>[2x]MGADDVVDSSKSFVMENFSSYHGTKPGYVDSIQKGIQKPKSGTQGNYDDDWEGFYSTDNKYDAAGYSVDNENPLSGKAGGVVKVTYPGLTKVLALKVDNAETIKKELGLSLTEPLMEQVGTEEFIKRFGDGASRVVLSLPFAEGSSSVKYINNWEQAKALSVELEINFETRGKRGQDAMYEYMAQACAGNRVRRSVGSSLSCINLDWDVIRDKTKTKIESLKEHGPIKNKMSESPNKTVSEEKAKQYLEEFHQTALEHPELSELKTVTGTNPVFAGANYAAWAVNVAQVIDSETADNLEKTTAALSILPGIGS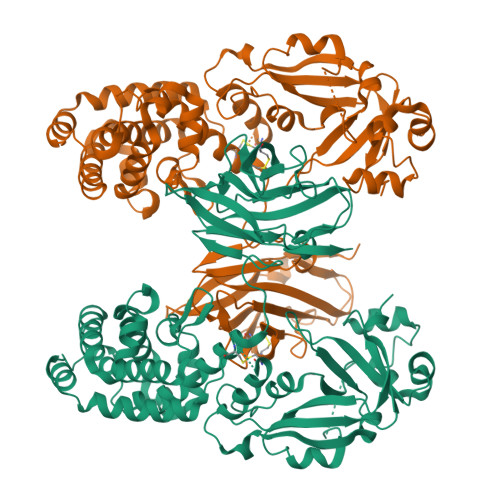VMGIADGAVHHNTEEIVAQSIALSSLMVAQAIPLVGELVDIGFAAYNFVESIINLFQVVHNSYNRPAYSPGHKTQPFLHDGYAVSWNTVEDSIIRTGFQGESGHDIKITAENTPLPIAGVLLPTIPGKLDVNKSKTHISVNGRKIRMRCRAIDGDVTFCRPKSPVYVGNGVHANLHVAFHRSSSEKIHSNEISSDSIGVLGYQKTVDHTKVNSKLSLFFEIKSMA> MSLQQVAVITLGIGDLEASARFYGEGFGWAPVFRNPEIIFYQMNGFVLATW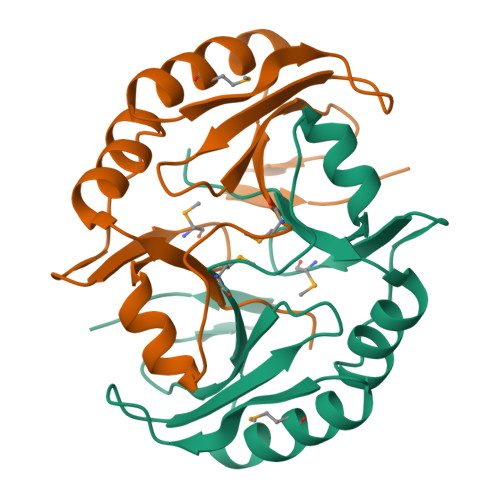LVQNLQEDVGVAVTSRPGSMALAHNVRAETEVAPLMERLVAAGGQLLRPADAPPHGGLRGYVADPDGHIWEIAFNPVWPIGADGSVTFAAKEGHHHHHH> MKRVLMGLILLSSSNITWAEAPSSKYQECLGRMTFEIPEEMEWATYDASRVWQISKGGGHNFTAEVTAVGDNGSYDYDSMIFYVSEKVDKNEFHNASNYIKGTAEIYQDHLRENIKLDKKAISTLQKNKSEEKSIERIKKGIAEMEAKIPLAKIYEHDLGIPDSHILGSKNIPFHVLLWRNQRVYYFTFSKPTENSAQRIKDLIARFRTRELYEVPNEPGICFPYGFIADDGKTAYELKNSLRFTRTPNVIFSLLTASANDPWQTRPTSGLYDSDFRPGYDRQKWKKSALLDSLHIGK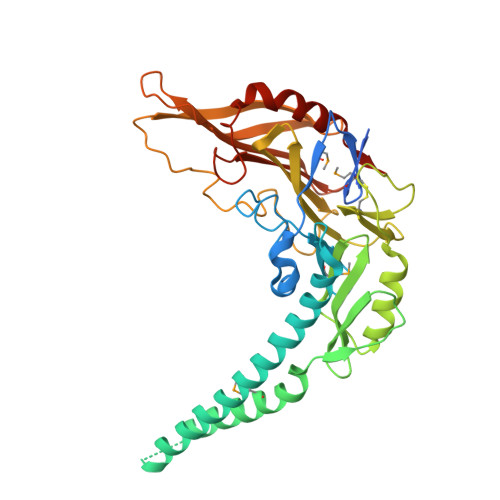RLAAFEGWRLDPRPDSGERERAWFGLAHTGGTLDPLVAIQVQTFQKGTDDLTDYTPPPEEVLPRLKALSQSIEQRLAR> EASIPTVERSTRMSNPWKAFMEKYDIERTHSSGVRVDLGEDAEVEN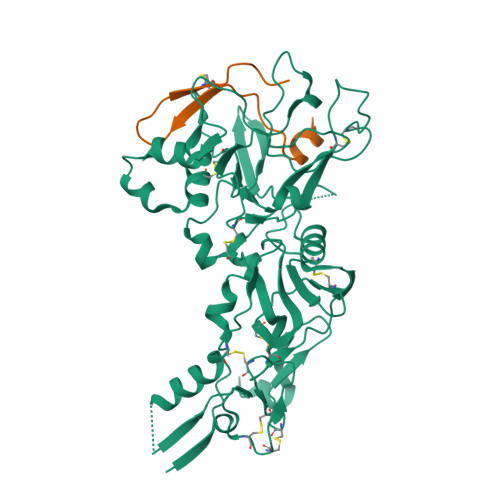AKYRIPAGRCPVFGKGIVIENSDVSFLRPVATGDEKLKDGGFAFPNANDHISPMTLANLKERYKDNVEMMKLNDIALCRTHAASFVMAGDQNSNYRHPAVYDEKEKTCHMLYLSAQENMGPRYCSPDAQNRDAVFCFKPDKDESFENLVYLSKNVRNDWDKKCPRKNLGNAKFGLWVDGNCEEIPYVKEVEAEDLRECNRIVFGASASDQPTQYEEEMTDYQKIQQGFRQNNREMIKSAFLPVGAFNSDNFKSKGRGFNWANFDSVKKKCYIFNTKPTCLINDKNFIATTALSHPQEVDLEFPCSIYKDEIEREIKKQSRNMNLYSVDGERIVLPRIFISNDKESIKCPCEPERISQSTCNFYVCNCVEKRAEIKENNQVVIKEEFRDYYENGEEKSNKQMLLLEQKLISEEDLNSAVDHHHHHH;> MDISQHATDIGMGPATSCYTSTIPPPKQVCIQQAVKATL>MEEPEEPADSGQSLVPVYIYSPEYVSMCDSLAKIPKRASMVHSLIEAYALHKQMRIVKPKVASMEEMATFHTDAYLQHLQKVSQEGDDDHPDSIEYGLGYLCPATEGIFDYAAAIGGATITAAQCLIDGMCKVAINWSGGWHHAKKDEASGFCYLNDAVLGILRLRRKFERILYVDLDLHHGDGVEDAFSFTSKVMTVSLHKFSPGFFPGTGDVSDVGLGKGRYYSVNVPIQDGIQDEKYYQICESVLKEVYQAFNPKAVVLQLGADTIAGDPMCSFNMTPVGIGKCLKYILQWQLATLILGGGGYNLANTARCWTYLTGVILGKTLSSEIPDHEFFTAYGPDYVLEITPSCRPDRNEPHRIQQILNYIKGNLKHVVIEGRGSHHHHHH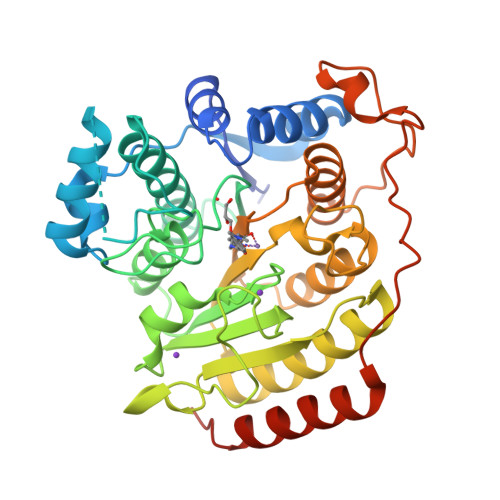[2x]>[8x]AGGKVTSSTGIAPKRYVYYPGSEELGPDEIRVIACGTGMPTARRAQAAAAWVVELGNGDKFIVDIGSGSMANIQSLMIPANYLTKIFLTHLATDHWGDLVSMWAGGWTAGRTDPLEVWGPSGSREDMGTKYAVEHMLKAYNWDYMTRAVTINPRPGDINVHEFDYRALNEVVYQENGVTFRSWPCIHAGDGPVSFALEWNGYKVVFGGDTAPNIWYPEYAKGADLAIHECWMTSDQMMTKYNQPAQLALRINLDFHTSAQSFGQIMNMVQPRHAVAYHFFNDDDTRYDIYTGVRENYAGPLSMATDMMVWNITRDAVTERMAVSPDHAWDVAGPSEDLAPDRNRASEYTQYILDGRLNVDEANAHWKQEFMG

PNGM-1 is derived from a metagenomic library from deep-sea sediments that predate the antibiotic era. PNGM-1 has both MBL and tRNase Z activities and is considered to be the evolutionary origin of B3 MBLs. The wild-type of PNGM-1 has two MBSs in its substrate-binding pocket, and each is occupied by a zinc ion. The zinc ion in the first MBS (Zn1) is coordinated by the residues His91, His93, His188, and Asp210; the zinc ion in the second MBS (Zn2), by Asp95, His96, His279, and Asp210.

His91 and His93 coordinate the zinc ion at Zn1, whereas His96 and His279 coordinate that at Zn2. In the H93A variant, the electron density for the zinc ion at Zn1 is weak to allow only a partial occupancy of a zinc ion or a full occupancy for a water molecule. The residues His93, Aps95, His279, and Asp210 occupy equatorial positions along the enzyme’s surface. In the structures of all PNGM-1 variants, except in that of H96A, the electron density corresponding to the catalytic water remains despite the complete or partial loss of a zinc ion. Each MBS of PNGM-1 is formed by four metal-coordinating residues, and the substitution of only one of these residues dramatically reduces the metal binding affinity of the enzyme.>MLIIGERINGMFGDIKRAIQERDPAPVQEWARRQEEGGARALDLNVGPAVQDKVSAMEWLVEVTQEVSNLTLCLDSTNIKAIEAGLKKCKNRAMINSTNAEREKVEKLFPLAVEHGAALIGLTMNKTGIPKDSDTRLAFAMELVAAADEFGLPMEDLYIDPLILPANVAQDHAPEVLKTLQQIKMLADPAPKTVLGLSNVSQNCQNRPLINRTFLAMAMACGLDAAIADACDEALIETAATAEILLNQTVYCDSFVKMFKTR[2x];>[2x]MPLTGLEIYKQLPKKNCGECGTPTCLAFAMNLASGKASLDSCPYVSDAAREALDAAAAPPIAKVVLGAGPTAVEMGDETELFRHDKRFYHETAIAIQVSDNLSSEELKAKVEAINGLNFDRVGQHYTIQAIAIRHDADDPAAFKAAVASVAAATQLNLVLMADDPDVLKEALAGVADRKPLLYAATGANYEAMTALAKENNCPLAVYGNGLEELAELVDKIVALGHKQLVLDPGARETSRAIADFTQIRRLAIKKRFRSFGYPIIALTTAANPLDEVLQAVNYVTKYASLVVLRTDAKEHLLPLLSWRQNLYTDPQVPIRVEEKLNEIGAVNENSPVYVTTNFSLTYYSVEGEIESTKIPSYLLSVDTDGLSVLTAYADGKFEAEKIAAVMKKVDLDNKVKRHRIIIPGAVAVLKGKLEDLTGWEVIVGPREASGIVAFARANLAS;>MAVQILRDRSRAAVQKVVLGATKDQGGTRSHTIVVGGDAALPFHHFEGEIVNRPVIGMEVQDIVPDWPDVLKDPFTDVINEPGRWAQKCVAEYGADLIYLKLDGADPEGANHSVDQC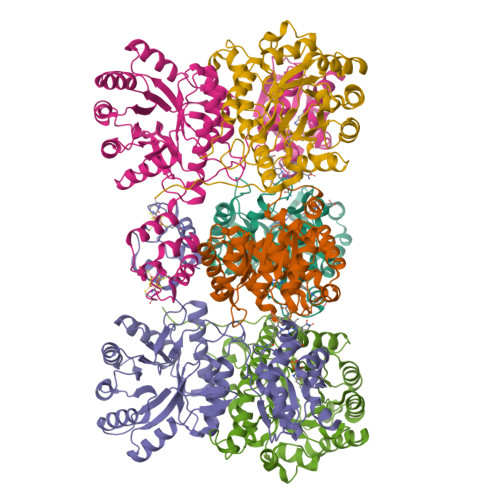VATVKEVLQAVGVPLVVVGCGDVEKDHEVLEAVAEAAAGENLLLGNAEQENYKSLTAACMVHKHNIIARSPLDINICKQLNILINEMNLPLDHIVIDPSIGGLGYGIEYSFSIMERIRLGALQGDKMLSMPVICTVGYEAWRAKEASAPVSEYPGWGKETERGILWEAVTATALLQAGAHILLMRHPEAVARVKENIDQLMVSNAY[2x]> MAHHHHHHAMQFDVTIEIPKGQRNKYEVDHETGRVRLDRYLYTPMAYPTDYGFIEDTLGDDGDPLDALVLLPQPVFPGVLVAARPVGMFRMVDEHGGDDKVLCVPAGDPRWDHVQDIGDVPAFELDAIKHFFVHYKDLEPGKFVKAADWV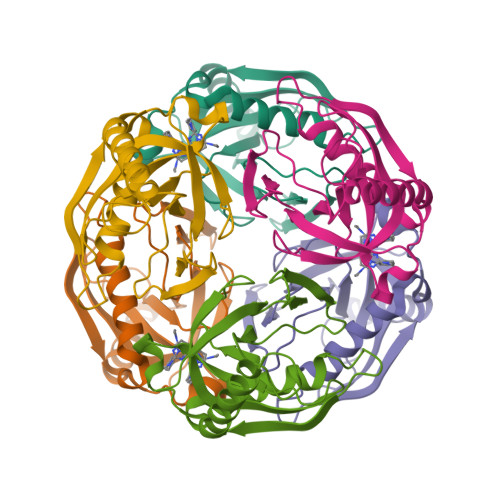DRAEAEAEVQRSVERFKAGTH>[2x]GSHMASMSQTPWWRGAVIYQIYPRSFLDSNGDGVGDLPGIIAKLDYISGLGVDAIWISPFFKSPMADFGYDISDYRAVDPLFGSLADFDRLLEKAHGLGLKVMIDQVLSHTSIAHAWFQESRQDRSNPKADWYVWADPREDGTPPNNWLSLFGGVAWQWEPRREQYYLHNFLVDQPDLNF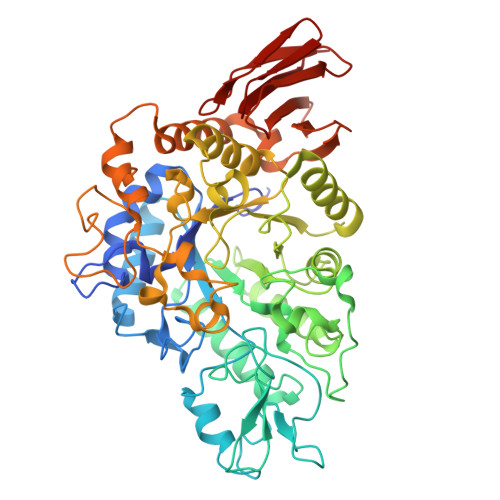HNAEVQQATLDNVRFWLDRGVDGFRLDAINFCFHDAQLRDNPAKPADKRVGRGFSADNPYAYQYHYFNNTQPENLPFLERLRGLLDSYPGAVSLGEISSEDSLATTAEYTAQGRLHMGYSFELLVQDYSAAYIRDTVSRLEATMLEGWPCWAISNHDVVRAVTRWGGAQATPAFARMVVALLCSLRGSICLYQGEELGLSEAEVAFEDLQDPYGITFWPTFKGRDGCRTPMPWTDAPSAGFTSGKPWLPLAASHRAAAVSVQQDDAHSVLRAVRAFLAWRKEMPALREGSIAFYDTAEPVLMFRREHAGQVVLLAFNLSADPAELALPAGEWEQIDVPGVELGAMDGGHLRLAGHAVVAAVGRG>[8x]MKIALVTHARHFAGPAAVEALTRDGYTVVCHDASFADAA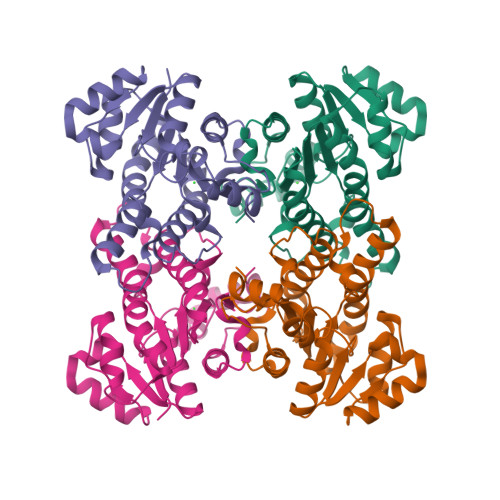ERQRFESENPGTVALAEQKPERLVDATLQHGEAIDTIVSNDYIPRPMNRLPIEGTSEADIRQVFEALSIFPILLLQSAIAPLRAAGGASVIFITSSVGKKPLAYNPLYGPARAATVALVESAAKTLSRDGILLYAIGPNFFNNPTYFPTSDWENNPELRERVERDVPLGRLGRPDEMGALITFLASRRAAPIVGQFFAFTGGYLP5-(3-fluoro-1H-pyrazol-4-yl)-2-[(naphthalen-2-yl)oxy]benzoic 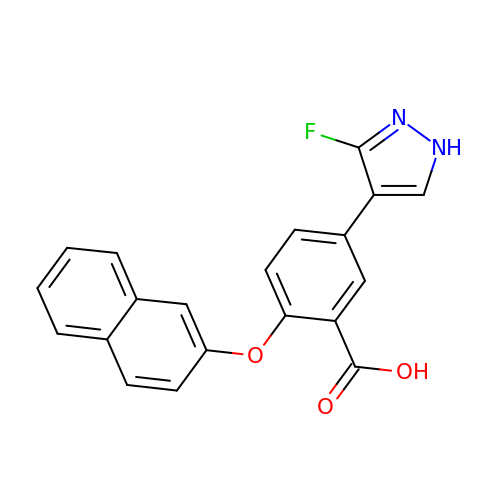acid | C20 H13 F N2 O3 | DLVKEINOBWQQLX-UHFFFAOYSA-N> THVDLGLASANVDFAFSLYKQLVLKAPDKNVIFSPLSISTALAFLSLGAHNTTLTEILKGLKFNLTETSEAEIHQSFQHLLRTLNQSSDELQLSMGNAMFVKEQLS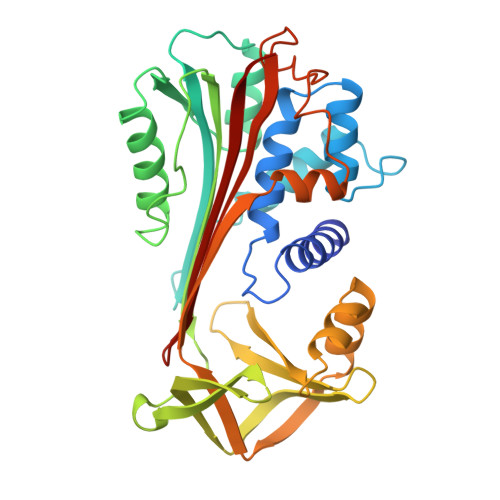LLDRFTEDAKRLYGSEAFATDFQDSAAAKKLINDYVKNGTRGKITDLIKDLDSQTMMVLVNYIFFKAKWEMPFDPQDTHQSRFYLSKKKWVMVPMMSLHHLTIPYFRDEELSCTVVELKYTGNASALFILPDQDKMEEVEAMLLPETLKRWRDSLEFREIGELYLPKFSISRDYNLNDILLQLGIEEAFTSKADLSGITGARNLAVSQVVHKAVLDVFEEGTERSAATAVKITLL ETHYL-(2-CARBOXY-4-GUANIDINIUM-PHENYL)-CHLOROACETATE | C12 H14 Cl 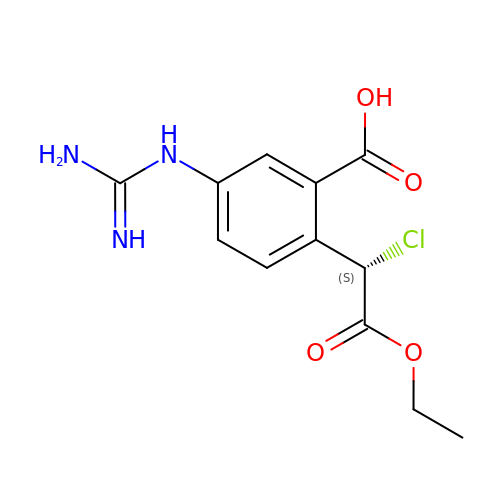N3 O4 | HIYFNBISGUASFH-VIFPVBQESA-N>GPGSASKAISDISLEVDRLGGRVSAFEMVTKKGGKIAEKDLVTVIELLMNELIKLDAIVAEGDVK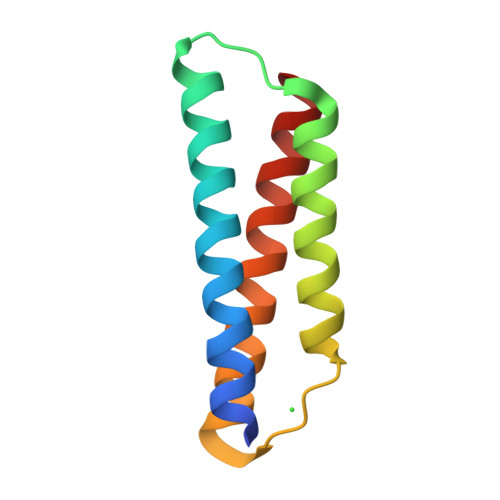LQRKMQVKRVQNYVETLDALKVKN[6x]>GMNGFSQLEGLRGHPSVVRVIGHRGARGVMPENTLEGFAFTLAAGVRALEFDVVMTADGVPVVTHNHHLANAMTRDGQGHWLTGAERQVAEMTYAEIRALDVGGLDGRTVYGRRFPDQAFLTGIHVPRLGELLDLCAGYGDQAPYLLLELKSDPALMHDHAARAEMVAAVLADVRRYRMEPRTVMHSFDWALLGECRRQAPDLPTSYLSQLPENADDPGEDSAKPVGPDYDRMTESLPQAVASAGGQLWCPYFLDVTPELVAEAHDLGLIVLTWTVNEPE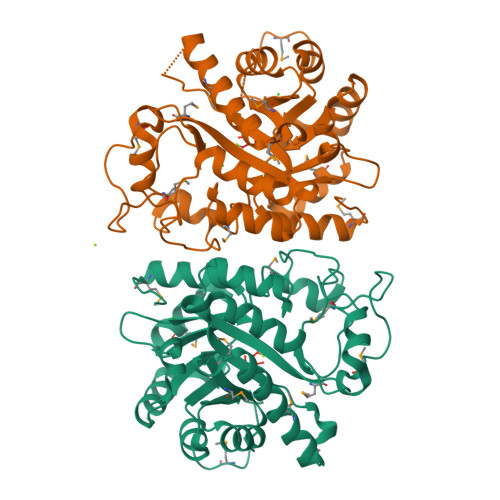DIRRMATTGVDGIVTDYPGRTQRILIDMGLSWT[2x]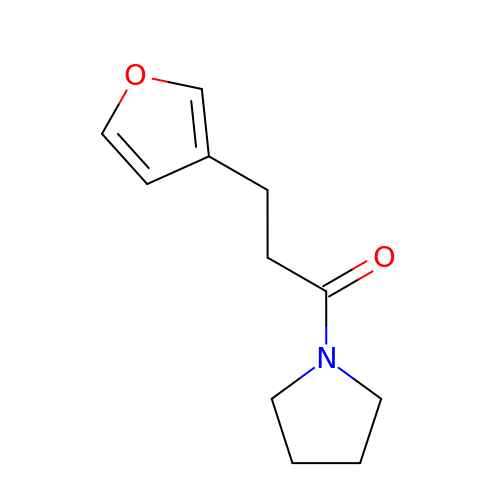3-(furan-3-yl)-1-(pyrrolidin-1-yl)propan-1-one | C11 H15 N O2 | SGKPSOSDSZDXFD-UHFFFAOYSA-N>[2x]APRKFFVGGNWKMNGDKKSLGELIHTLNGAKLSA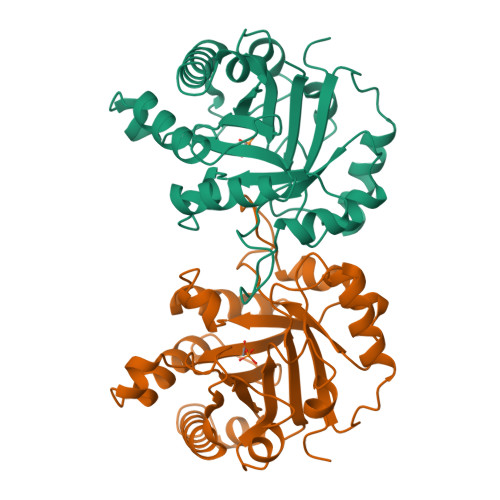DTEVVCGAPSIYLDFARQKLDAKIGVAAQNCYKVPKGAFTGEISPAMIKDIGAAWVILGHPERRHVFGESDELIGQKVAHALAEGLGVIACIGEKLDEREAGITEKVVFEQTKAIADNVKDWSKVVLAYDPVWAIGTGKTATPQQAQEVHEKLRGWLKTHVSDAVAQSTRIIYGGSVTGGNCKELASQHDVDGFLVGGASLKPEFVDIINAKH> MSLKFPDTGLEEKEVAFSIVNHAAKSLGFIHVDQWDYERVMFDYKIVHHEGTFYL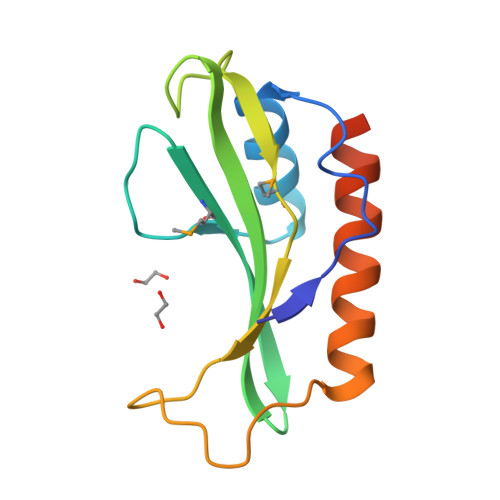RVPAYAVKGEIPRPSTIVQIMTPILGKYYYPHGVEYEGETFPQAVIDKCNNKLALLAKTIKAEWEGHHHHHH> MDSTNLNKRPLLQYSLSSLGSQITKWSSSRPTSPVRKARSTENDFLSKQDTSSILPSINDDGGEQWYEKFKPNCLEQVAIHKRKLKDVQEALDAMFLPNAKHRILLLSGPSGCSKSTVIKELSKILVPKYRQNSNGTSFRSTPNEHKVTEFRGDCIVNDLPQMESFSEFLKGARYLVMSNLSLILIEDLPNVFHIDTRRRFQQLILQWLYSSEPLLPPLVICITECEIPENDNNYRKFGIDYTFSAETIMNKEILMHPRLKRIKFNPINSTLLKKHLKFICVQNMKMLKEKNKWNKRQEVIDYIAQETGDIRSAITTLQFWATSSGSLPISTRESTISYFHAIGKVIHGSHSTNNDNEMINNLFENSNNLLSKEDFKLGILENYNTFNKGEFSISDASSIVDCLSECDNMNGLPESNEYGLREVRKTFRNISKQGHNHGTVYFPREWKVRKLQNSFKVQAEDWLNVSLYKYNAVHSFRNITLEFGYYAPLIRKCQSYKKKYILYYLKNLPSGSSGPKQTMDKFSDIMKVENGIDVVDRIGGPIEALSVEDGLAPLMDNDSNNCDHLEDQKKERDRRLRMLIDQYERNVMMANDDLEDEETSFNDDPIVDSDSDNSNNIGNETFGRSDEDESLCEILSQRQPRKAPVISESLSDSDLEILGLNLEVLFQGPGGDYKDDDDKDYKDDDDKDYKDDDDK;> MSKTLSLQLPWVEKYRPQVLSDIVGNKETIDRLQQIAKDGNMPHMIISGMPGIGKTTSVHCLAHELLGRSYADGVLELNASDDRGIDVVRNQIKHFAQKKLHLPPGKHKIVILDEADSMTAGAQQALRRTMELYSNSTRFAFACNQSNKIIEPLQSRCAILRYSKLSDEDVLKRLLQIIKLEDVKYTNDGLEAIIFTAEGDMRQAINNLQSTVAGHGLVNADNVFKIVDSPHPLIVKKMLLASNLEDSIQILRTDLWKKGYSSIDIVTTSFRVTKNLAQVKESVRLEMIKEIGLTHMRILEGVGTYLQLASMLAKIHKLNNKA;> MSTSTEKRSKENLPWVEKYRPETLDEVYGQNEVITTVRKFVDEGKLPHLLFYGPPGTGKTSTIVALAREIYGKNYSNMVLELNASDDRGIDVVRNQIKDFASTRQIFSKGFKLIILDEADAMTNAAQNALRRVIERYTKNTRFCVLANYAHKLTPALLSRCTRFRFQPLPQEA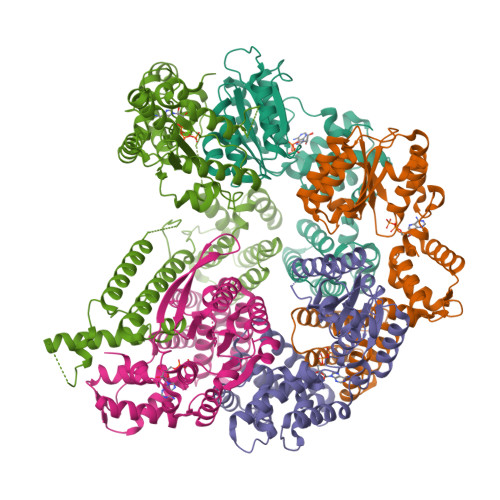IERRIANVLVHEKLKLSPNAEKALIELSNGDMRRVLNVLQSCKATLDNPDEDEISDDVIYECCGAPRPSDLKAVLKSILEDDWGTAHYTLNKVRSAKGLALIDLIEGIVKILEDYELQNEETRVHLLTKLADIEYSISKGGNDQIQGSAVIGAIKASFENETVKAN;> MFEGFGPNKKRKISKLAAEQSLAQQPWVEKYRPKNLDEVTAQDHAVTVLKKTLKSANLPHMLFYGPPGTGKTSTILALTKELYGPDLMKSRILELNASDERGISIVREKVKNFARLTVSKPSKHDLENYPCPPYKIIILDEADSMTADAQSALRRTMETYSGVTRFCLICNYVTRIIDPLASRCSKFRFKALDASNAIDRLRFISEQENVKCDDGVLERILDISAGDLRRGITLLQSASKGAQYLGDGKNITSTQVEELAGVVPHDILIEIVEKVKSGDFDEIKKYVNTFMKSGWSAASVVNQLHEYYITNDNFDTNFKNQISWLLFTTDSRLNNGTNEHIQLLNLLVKISQL;> MSLWVDKYRPKSLNALSHNEELTNFLKSLSDQPRDLPHLLLYGPNGTGKKTRCMALLESIFGPGVYRLKIDVRQFVTASNRKLELNVVSSPYHLEITPSDMGNNDRIVIQELLKEVAQMEQVDFQDSKDGLAHRYKCVIINEANSLTKDAQAALRRTMEKYSKNIRLIMVCDSMSPIIAPIKSRCLLIRCPAPSDSEISTILSDVVTNERIQLETKDILKRIAQASNGNLRVSLLMLESMALNNELALKSSSPIIKPDWIIVIHKLTRKIVKERSVNSLIECRAVLYDLLAHCIPANIILKELTFSLLDVETLNTTNKSSIIEYSSVFDERLSLGNKAIFHLEGFIAKVMCCLD>[2x]MNDLEKLVELLTHDDSKTQQEAARDLAEIASGNASAIKQVIDAGALEKLVELLTHDDSKVQQEAARALANIASGNDEAIKQVIDAGALEKLVELLTHDDSKVQQEAARALANIASGNDEAIKQVIDAGALEKLVELLTHDDSKVQQEAARALANIASGNDEAIKQVIDAGALEKLVELLTHDDSKVQQEAARALANIASGNTSAIKQVIDAGALEKLQELLTHDDSKVQQEAQRALENIK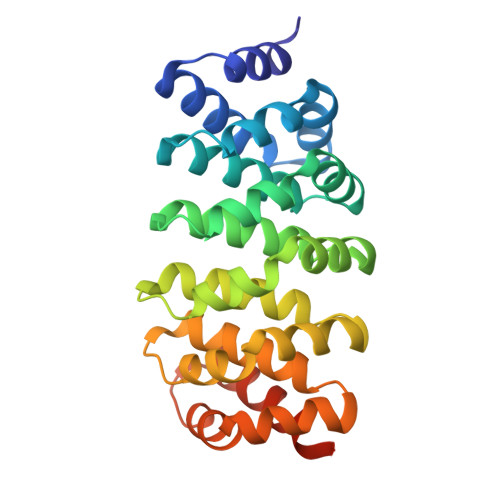SGGWLEHHHHHH> H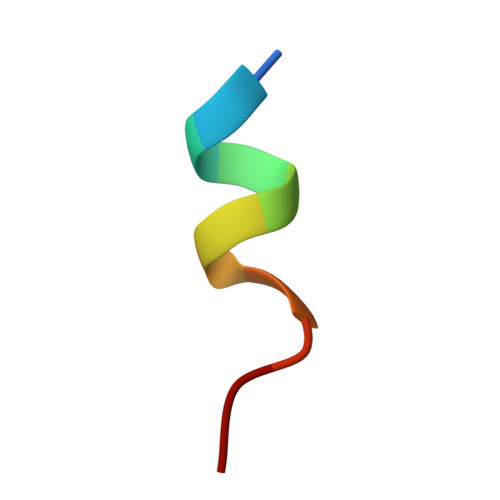KILHRLLQDS> SSIHEVVALIEELYSPHPKHDVNQIQQSLQSIQKSEQGFHLANELLSDDKYSANVKYFGALTLTVQLNTRGENDYETLWNVFRSNLLYLTKFSTLYVSNPNMY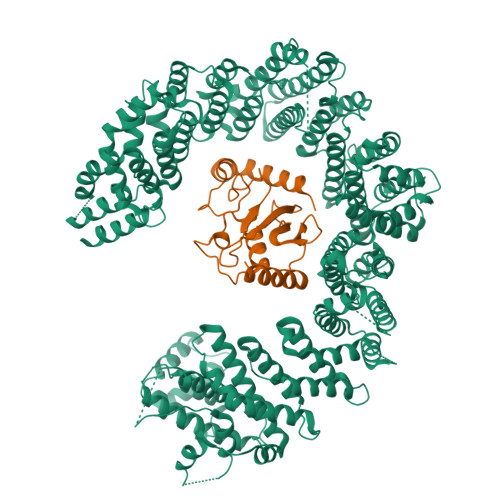GQSLIIIKKLMSNLSLIFTKINDPQLNNAGNENMIKQWNNPINTFIQLMSVQNQNINADQLLLDSINCSLTYEQLSQFVSLSQKHNELALTFTEVIVEDLTKFQTKRHSMSQIHEVVHEHLYISTMALINLNLTAQAVFNPTVFDCITAWINYISLTRSVSSSGRMDLSEIFQNLIDLMYQSTEGSDGYENAEKILTIFGNVFANDPLLMSYDLRQQIECIFLGVVRPDSGITDISNKNSWMLQYMNYLVTNDFFSELKELAICIVDFLQINTLSVCNKLFTNIQAADNGQVQDEYIQEYIKVLLQMTNFPLTPVLQEFFSVRMVDFWLDLSDAYTNLASETLRPNSIELSTQIFQQLINIYLPKISLSVKQRIIEEEGESTSVNEFEDFRNAVSDLAQSLWSILGNDNLTNVLIDGMGQMPAASDETLIIKDTDVLFRIETMCFVLNTILVDMTLSESPWIKNIVDANKFFNQNVISVFQTGFQTSASTKVSQILKLDFVRTSTTLIGTLAGYFKQEPFQLNPYVEALFQGLHTCTNFTSKNEQEKISNDKLEVMVIKTVSTLCETCREELTPYLMHFISFLNTVIMPDSNVSHFTRTKLVRSIGYVVQCQVSNGPEEQAKYILQLTNLLSGSIEHCLASSVQLQEQQDYINCLLYCISELATSLIQPTEIIENDALLQRLSEFQSFWSSDPLQIRSKIMCTIDKVLDNSIYCKNSAFVEIGCLIVGKGLNLPDGEPYFLKYNMSEVMNFVLRHVPNCELATCLPYFVYLLEKLISEFRKELTPQEFDFMFEKILLVYYDAYIINDPDLLQMTIGFVNNVLDVKPGLAIGSKHWTSFILPQFLKLIPSREKFTIVAVAKFWTKLINNKKYNQEELTTVRQQVSSIGGDLVYQIMYGLFHTQRSDLNSYTDLLRALVAKFPIEAREWLVAVLPQICNNPAGHEKFINKLLITRGSRAAGNVILQWWLDCTTLPNYQG;> GSSLCLQRLQEERKKWRKDHPFGFYAKPVKKADGSMDLQKWEAGIPGKEGTNWAGGVYPITVEYPNEYPSKPPKVKFPAGFYHPNVYPSGTICLSILNEDQDWRPAITLKQIVLGVQDLLDSPNPNSPAQEPAWRSFSRNKAEYDKKVLLQAKQYSK> GSHMASMSKDEVKREAKDTDGNPEIKGERRRLHSEIQSTSLANNIKKSTVIVKN;> PTHIAICLYYKLGETPLPLVIETGKDAKALQIIKLAELYDIPVIEDIPLARSLYKNIHKGQYITE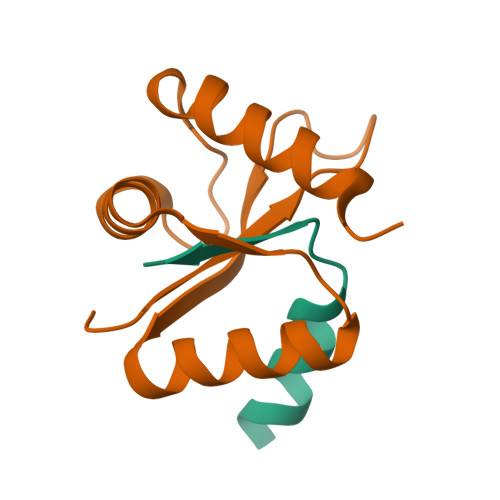DFFEPVAQLIRIAIDLDY> Y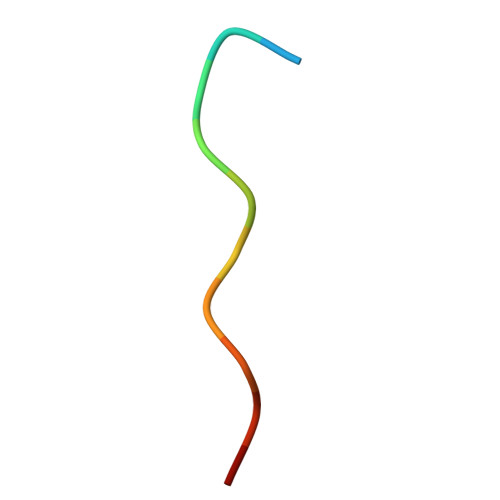EVPGPVPPRRR3~{H}-pyrrolo[2,3-c]isoquinolin-5-amine 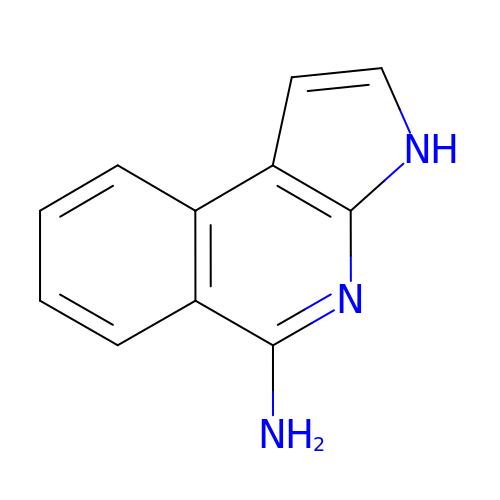| C11 H9 N3 | OEJVERPJEZHNRW-UHFFFAOYSA-N> GSHMPRDYTPICDNIVKLTLTSDGKSITLYGLQYGNYIITNRHLFRLNNGTLTIESKNGTYTIADSKTLEVHLIEGKDLVILKMPDSVPAADTTLKFKKPVENEEVVLVSRDFSTPEPKCLVSESSKITPDNDGTFWKHSIPTKDGE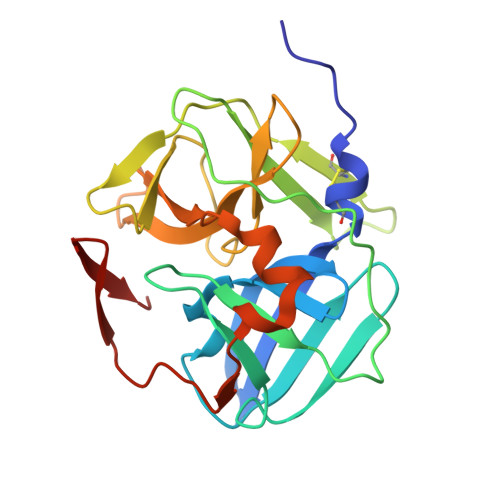AGLPLVSTKDGTVVGLHSASNFNNTNFYFTAIPENFMELLNDESKRKWIKGWHLTSNSVEWGGHKVFMDK> ATIKDVAKRANVSTTTVSHVINKTRFVAEETRNAVWAAIKELHYSPSAVARSLKVNHTKSIGLLATSSEAAYFAEIIEAVEKNCFQKGYTLILGNAWNNLEKQRAYLSMMAQKRVDGLLVMCSEYPEPLLAMLEEYRHIPMVVMDWGEAKADFTDAVIDNAFEGGYMAGRYLIERGHREIGVIPGPLEQNTGAGRLAGFMKAMEEAMIKVPESWIVQGDFE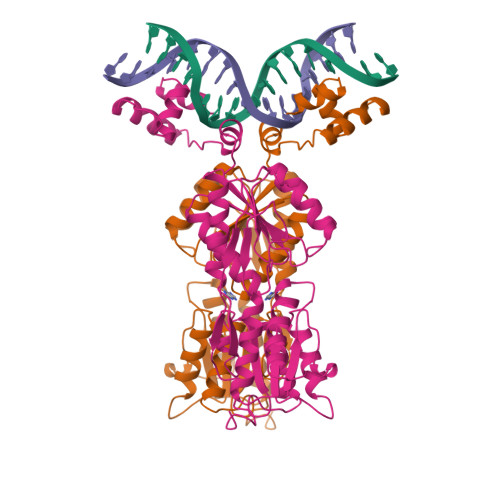PESGYRAMQQILSQPHRPTAVFCGGDIMAMGALCAADEMGLRVPQDVSLIGYDNVRNARYFTPALTTIHQPKDSLGETAFNMLLDRIVNKREEPQSIEVHPRLIERRSVADGPFRDYRR>[2x]MIDLIVSQGRVADRAAWMIEGAARTARALEERYGLKGHYVGEPAPHADDDWSVALPQARETLVAVREAATESIKGDNLTVLVNNTCSV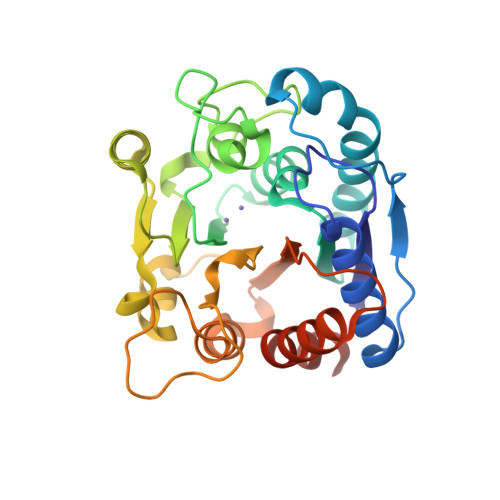SLATLPVVAREHPDAVVLYIDGHGDFNTPETTDTGYLGGMVLSGACGLWDSGHGAGLRPEQAVLVGSRDIDEGERELIRKAGVRVIPPGEATAQAVLDAVKDAPVWIHIDWDVLEPGSIPADYTVPDGMLPAQIRAVFEAIPAERLIGVELAELNAPADSERAEQAVAVILDMVAPAFDAAAARPLEHHHHHH>[2x]MSQSNRELVVDFLSYKLSQKGYSASGGGGGGGMAAVKQALREAGDEFELRYRRAFSDLTSQLHITPGTAYQSFEQVVN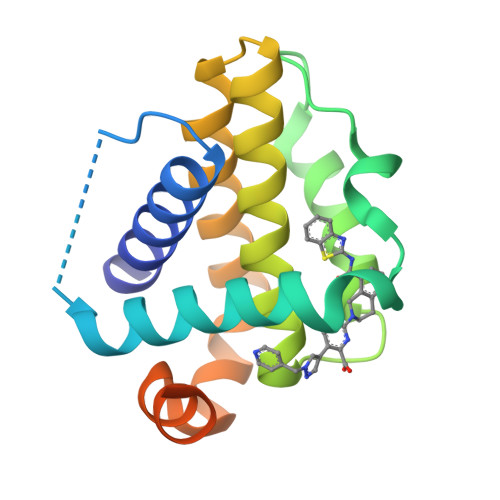ELFRDGVNWGRIVAFFSFGGALCVESVDKKMQVLVSRIAAWMATYLNDHLEPWIQENGGWATFVELYGNNAAAESRKGQERLEHHHHHH>GSMTWNFHQYYTNRNDGLMGKLVLTDEEKNNLKALRKIIRLRTRDVFEEAKGIAKAVKKSALTFEIIQEKVSTTQIKHLSDSEQREVAKLIYEMDDDARDEFLGLTPRFWTQGSFQYDTLNRPFQPGQEMDIDDGTYMPMPIFESEPKIGHSLLILLVDASLKSLVAENHGWKFEAKQTCGRIKIEAEKTHIDVPMYAIPKDEFQKKQIALEANRSFVKGAIFESYVADSITDDSETY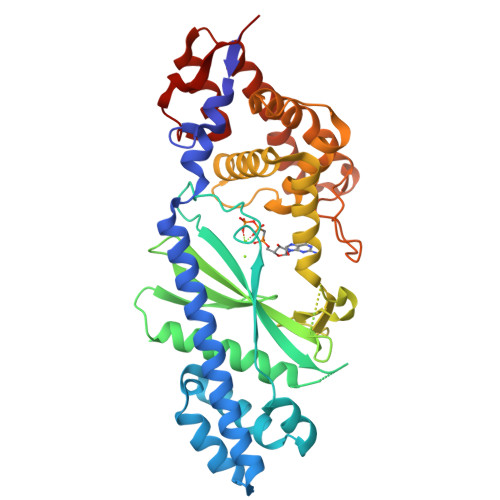ELDSENVNLALREGDRKWINSDPKIVEDWFNDSCIRIGKHLRKVCRFMKAWRDAQWDVGGPSSISLMAATVNILDSVAHDASDLGETMKIIAKHLPSEFARGVESPDSTDEKPLFPPSYKHGPREMDIMSKLERLPEILSSAESADSKSEALKKINMAFGNRVTNSELIVLAKAL[2x]> MKVTKSEIVISAVKPEQYPEGGLPEIALAGRSNVGKSSFINSLINRKNLARTSSKPGKTQTLNFYIINDELHFVDVPGYGFAKVSKSEREAWGRMIETYITTREELKAVVQIVDLRHAPSNDDVQMYEFLKYYGIPVIVIATKADKIPKGKWDKHAKVVRQTLNIDPEDELILFSSETKKGKDEAWGAIKKMIN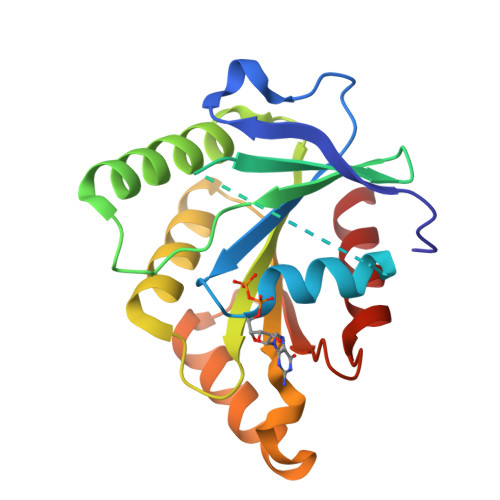R>[2x]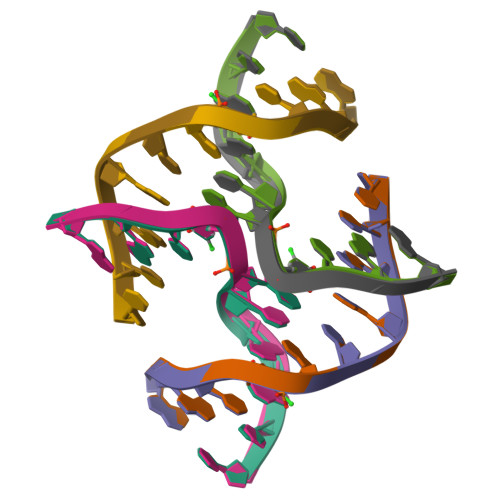CCGATACCGG;>[2x]CCGGTAUCGG> MHHHHHHTLFGDVSGKGAPLNAARPAEERAALLAWVKERLHEEYGDQDPTPRRDPMHELISTILSQRTTHADEEAAYQELRTLGDWDAITLAPTDAVAHAIRRSNYPESKAPRIQETLRRIKAAPGGYDLDFLRDLPVKDALKWLTDLPGVGVKTASLVLLFNYARPVFPVDTHVHRVSTRVGVIPRMGEQAAHRA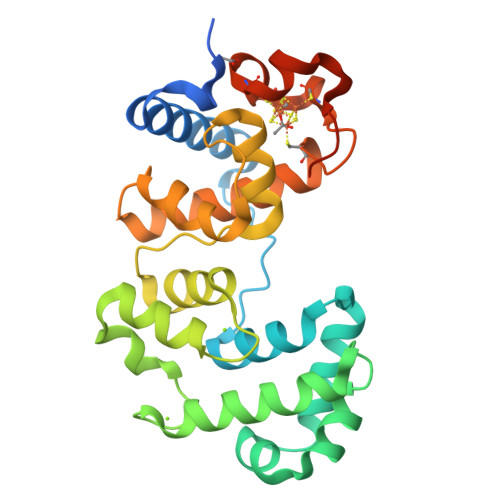LLALLPPDPPYLYELHINFLSHGRQVCTWTRPKCGKCILRERCDAYALYGDKVPSFSEKPVKGEKPAKG>KKNGYAVDSS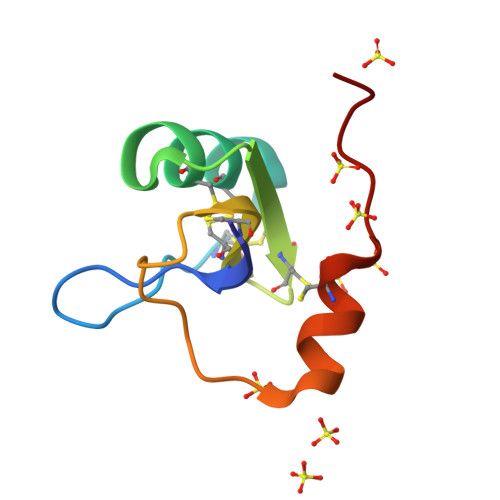GKVAECLFNNYCNNECTKVYYADKGYCCLLKCYCFGLADDKPVLDIWDSTKNYCDVQIIDLS[2x]> MVKLNCRPLCQAPTASRLVSPP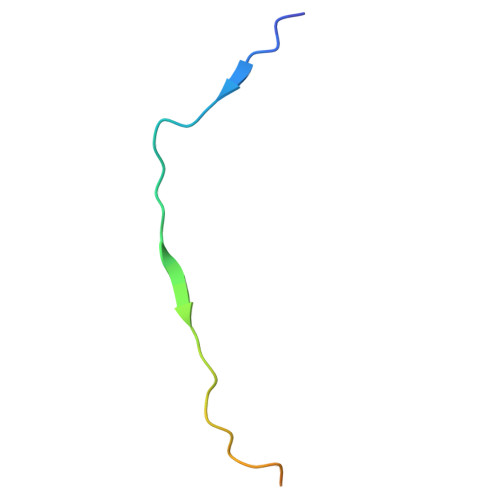CFICRGVAPSAPVTPG>SGSIEALMLFGSAARGESDKNSAVALLAVTSGVRPFSKKTEQTELQFLNPEELLRSASDGDLFAIHLAFEGKIIFDTTGVFTRFKERLVIRKDYGREIKWGNDLAWYLLDFGMNAENTTLVNKRIAWCVRTIAIARLVESGKIIFSPRALAKEFPRKHVSDLIGLRRSDEDSQTRKRRLAGFLD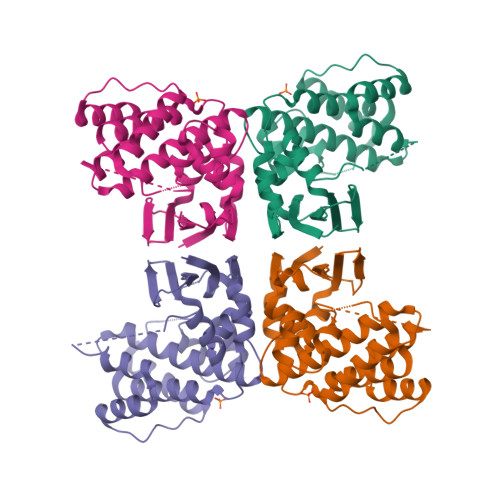SIDSSRPSVSSEQEYVSHFERTENRVGLQTLHGLKKKNGNEESPY[4x]> GSSGSSGDDKRGRREIRVLHLLEQIRAYCETCWEWQEAHEPGMDQDKNPMP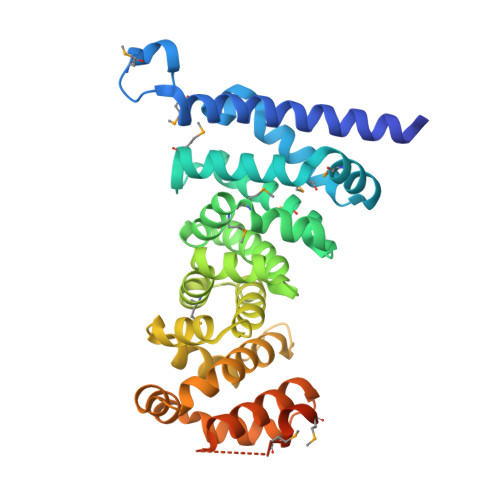APVEHQICPAVCVLMKLSFDEEHRHAMNELGGLQAIAELLQVDCEMYGLTNDHYSITLRRYAGMALTNLTFGDVANKATLCSMKGCMRALVAQLKSESEDLQQVIASVLRNLSWRADVNSKKTLREVGSVKALMECALEVKKESTLKSVLSALWNLSAHCTENKADICAVDGALAFLVGTLTYRSQTNTLAIIESGGGILRNVSSLIATNEDHRQILRENNCLQTLLQHLKSHSLTIVSNACGTLWNLSARNPKDQEALWDMGAVSMLKNLIHSKHKMIAMGSAAALRNLMAN> A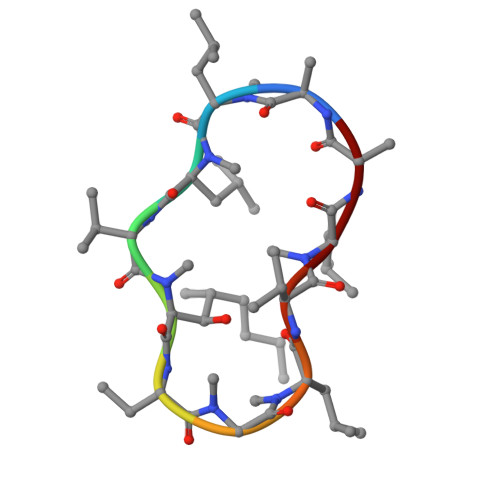LLVTAGLVLA>MSEPMMWLLVRGVWETLAMTFVSGFFGFVIGLPVGVLLYVTRPGQIIANAK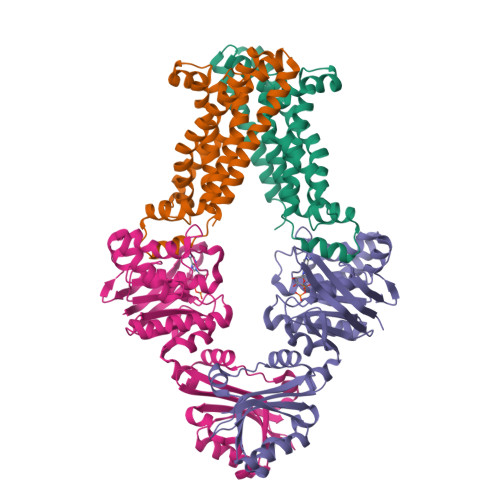LYRTVSAIVNIFRSIPFIILLVWMIPFTRVIVGTSIGLQAAIVPLTVGAAPFIARMVENALLEIPTGLIEASRAMGATPMQIVRKVLLPEALPGLVNAATITLITLVGYSAMGGAVGAGGLGQIGYQYGYIGYNATVMNTVLVLLVILVYLIQFAGDRIVRAVTRK[4x];>MGHHHHHHHHHHSSGHIDDDDKHMIKLSNITKVFHQGTRTIQALNNVSLHVPAGQIYGVIGASGAGKSTLIRCVNLLERPTEGSVLVDGQELTTLSESELTKARRQIGMIFQHFNLLSSRTVFGNVALPLELDNTPKDEVKRRVTELLSLVGLGDKHDSYPSNLSGGQKQRVAIARALASNPKVLLCDQATSALDPATTRSILELLKDINRRLGLTILLITHEMDVVKRICDCVAVISNGELIEQDTVSEVFSHPKTPLAQKFIQSTLHLDIPEDYQERLQAEPFTDCVPMLRLEFTGQSVDAPLLSETARRFNVNNNIISAQMDYAGGVKFGIMLTEMHGTQQDTQAAIAWLQEHHVKVEVLGYV[4x]> MLNVLSSTASAALATVVVARPSALHLIFERCKLNLVEFTAQDVYQICTTAYNMDTLGMLQDPDFMRGLHDAFRRSDQTVISPFQANLIADTFRKVGINSMPKEVSVPEEDAISPESLILVLRNMNITKQRDERKINEVLKLMFPILDEFSPTQLSLTVTELARLKSTNADFVGKLAKRIMEYNDDLSALDISSAAVSLAYCPGISHNILYRMMQIVEERMGEFQPEDYINVLHALNTLGPKFVNTFRKIVECGLQHVENMDAVTLTNYMVCFSTMDYKQREHIDIYADALVEVATDLSEKDLVMAFIALQRLRLLSDTMFGTMASCVIRYAAKMDPRNIAPIMDICSTVPHASDHLMKVLMDRAVECTRILTANQLGDILDILGLYPPAREHPLVQLFGKQARLRLDLMGPDALANATRGLANLGYADPEYYAQAAETGFRYGFKDWTLLEPMLMGLSITGQCPPTMVRVLGSHIAPMARSMSLMEIERANRYLRRLGCEDDFVYKAMASRVLQ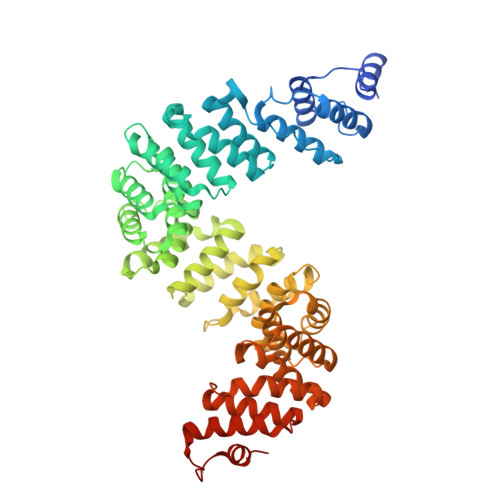FVKEVTPEMPEDLQVLLQRGAVEPGAAPGVM>[3x]MRRFGSKFASGLASRCALACPLASAATAPAGASTTSSTSSAQKSFFKTTEMIGYVHSIDGTIATLIPAPGNPGVAYNTIIQIQVSPTTFAAGLVFNLEKDGRIGIILMDNITEVQSGQKVMATGQLLHIPVGAGVLGKVVNPLGHEVPVGLVTRSRRLLDSTLGKVDTGAPNIVSRSPVNYNLLTGFKAVDTMIPIGRGQRELIVGDRQTGKTSIAVSTIINQVRINQQILSKNAVISIYVSIGQRCSNVARIHRLLQSYGALRYTTVMAATAAEPAGLQYLAPYAGVTMGEYFMNRGRHCLCVYDDLSKQAVAYRQISLLLRRPPGREAYPGDVFYLHSRLLERAAMLSPGKGGGSVTALPIVETLSNDVTAYIVTNVISITDGQIYLDTKLFTGGQRPAVNIGLSVSRVGSSAQNAAMKGVAGKLKGILAEYRKLAADSVGGQQVQTIPMIRGARFVALFNQKQPSYFMNAIVSLYACLNGYLDDVKVQYVKFYEYLLVHRDLGIMYGTAKNKFFYMYVQELNYLIRFFTLNSPILHGELEEMLKQHTHLFLQHYQSKMNAIKSEKDVKALKNLLYSCKRAV;>[3x]MLTRFRSAVLRGAVSITGARAASTAPVADHKGRVGHVSQVIGAVVDVHFADGVPPVLTALDVVDKLGRDEPLTLEIVQHLDAHTGRCIAMQTTDLLKLKAKVVSTGGNISVPVGRETLGRIFNVLGDAIDQRGPVGEKLRMPIHAVAPKLADQAAEDAVLTTGIKVIDLILPYCKGGKIGLFGGAGVGKTVIIMELINNVAKGHGGFSVFAGVGERTREGTDLYLEMMQSKVIDLKGESKCVLVYGQMNEPPGARARVAQSALTMAEYFRDVEGQDVLLFIDNIFRFTQANSEVSALLGRIPAAVGYQPTLAEDLGQLQERITSTTKGSITSVQAVYVPADDITDPAPATTFSHLDATTVLDRAVAESGIYPAVNPLECASRIMDPDVISVDHYNVAQDVVQMLTKYRELQDIIAVLGIDELSEEDKLIVDRARKLVKFLSQPFQVAEVFTGMTGHYVQLDDTIDSFSGLLMGTYDQVPEMAFYMVGGINSVLEKAKKMAEEAAELEKMRRARVAQASS;> MSGKLRLYKEKLEGYNRFYSIVKTIKMVTLAKYRAAQGRIRTRDFSLRYTELAFSKPQASRDAVVAAKNALVYIPITTNRGSCGALNSNIVRCIDSVVSSKMVLMPVGKRGIDSFSKLYPDEFRYGIINDMKESMHFGYATFVIENAYEVSKDADRYQVIFNRFVSAGVQRNAVYNIPSYEKWKEDLADAASSDNQKNRYLFANALQNEEEQLIRDFFDFHAALAVLNAVGENELSEQAARLVAVEGQLTNISSLQQRTSSLYNKTRQFGITAALIEILSAMSSLEGNAMKGVRRNKFWEGAVTK;> MFRTFGRRLVSCTLPLLQSAPHDLPEGFEFMEHKVVNKDIHAPHENLETLRLTLTRQDEFLLREEPVKCVTVTGTNGEYGIYPGHAYKIVQLNPSPLTVEYTDGTTKKYFVSGGFAHINNEGSCDVNTVECTLLDDLDLAIAEKELAAQQAALGSAKDDKAKSVVEIRISVIEAVIAALKHH;> MIRRSCALLSSSWRDHGISYLKYLNVCTETLHSTVKESRRAKYERWSKPCYTAQRPDGAGGQETIDKVPIHTKDY;>[3x]MMRRVYSPVFCSVAAARFAATSAAKKYDLFGYEVDTNTAPWIEKIKKCKYYDEAGEVLVNMNVSNCPPDIATYNATLQCIYQSPSKQSTPVDNESKFCAMMDLLEEMQHRNRLKPNEESWTWVMKECVKSGQFRLGYCIQQVMETECKGCPADLVKANEANAQKAKTEGKEHPGHLSQQAGLFDVKVE;>MSAKAAPKTLHQVRNVAYFFAAWLGVQKGYIEKSANDRLWVEHQRKVRQQNVERQQALDSIKLMQQGVRATTPGQLEGVPAELQQLAEAFTK[2x];>[2x]MSSTKCAVACKIMTPLCNAASKVQARSAKKLAALTDAGIQKTISEHNANGTDAAVSSTKRYLAEQRQLFHYRVVRFFDECHYIISGEYFAQYTKVNLIWDLRFLTKLVVLFLIGTVLGRQSIFPPIDPDSPLVEALVTKVNPNY;> MFRRLSSSARAVVAARFYTPPEGLKKLYASDFENSKYPLNIVPSDSVLFAKFLYKAAEEKGNFDNILSDFQKIAAAASKLPIFWERTAVVEKIPEFKQLSEPTFFTLVWMQNNGMLELIQEVAEVYETFVNAKQKKAVAKIFVAPGGEKNVEEARRVAEELHKGLKELADYTLVLKTVVDRTIVKGFAVELAGQYVNKAEGQQKQAGRADEVDYTNLPAPKPQKTVWDDNIETEVLRKYLDGLSQYDMEEAKYGV;>MMRRLALQSSIRRATPFATPLVASTKALNPMCSAITIREASTVAISVQGLHYVGTGLAAIALAGVGLGIGTIFGNLLVACARQPNLTKMLFNYAILGFALTEAIGLFALMLAFLMLFS[10x];> MFLFFFCDLFWLRLLLCMYYCVWSRLCFIVYFNCLMLIFDFLLFCLFDLYLFVGLCLFLLLWFMLFNLYSLILYYCITYLNLYLLFCIVFLLYIAFLFLFCFLCDFFLFNNLLVGDSFMDVFFIRFLLCFLECFSLLCRCLSTFLRLFCNLLSSHFLLLMFFDFFYFIFVFFFYGVFCYWFILFIFVFCFCLLFYVFLYLLDLFAAILQLFIFCNMILQLIMDFLLFLLFV;> MLRRLGANVSNMARPMNKYAVTVSPRRHLEPMSTWYLASWAMVWYYAFFFWMPMVWTDIMVPSFVYNKLPVIHFLQEKRAEQKLRRVLDETYTEWTEELDQAHVTDAITRSLNI;> MRRVSSPNITIQSVRWISGVSPLLYFPPTTTSTTNREDQINKNTNIAIQMIKRYKGEVPPHYTRKSSATIEQVEKEIDALLGGAEKLRKTSTDDQPMDKLTLMERCLRHALWSYHKEEGRYDFDQIGRWVVYTPEDEVKLAQLKREVEAKEKLAALRKRREEEGLPGGPVPRINWPQEYSSFIDREPVVAKRIRYDTLASTTLERDEKQIESTLQQYRRASQDKRLDDLVDLLERFKPVLAREAIMQRLTIKHLEGQLGVWRYMDWCPEVRDRAELEVDITGWQWWSPLEERRLLPVRLRSVNEVREIMSKTQAKKSAEAAERNPIVTQTSTGDNARDRLLKEVLALQARINQRDEVEPSQTEQKKKAHH;> MQGSWSVLKKNCSNFFPGLLAFAQQTQEAYGIWLRIYNRQQKYGPTDFVEQSETFSPDYHKRFHSQDKNMWVDKELCTEVSQKEVARLMTYKLDMWRMAHCAGALLATGGYAIPFGLFWLANDTWVPSSFNLTGEELRAWREAQDLYRYRSAPSYLTDTKWHFDFHAYPWNETQERAWDDLFEKNDVRRDPKVVRPAAEMYDGFIKFELIRRKSLRHLCRSMNIPTFPMLARLCNGTRVRDYWNLAWCEDYMVITQRLHESMTDEELYDYAWRRYLAPYDKNLNREQLMERVEDYFEFLGPDFVAHGKAPNLVILTNYVLGYYNDPAYLEGDISELDKNDYDHLASWGKDAFLRRLEFENGPLRDQVEAHTQRLLAERAAIAKGDNAAAVEGRHTA;> MVLFSTYRSSRLVSKEFLHGPVMRFRALGEYYFQRAWNGTLNWALPGEYRLYAVMIPFIYFYHRWHNDHTLDRDHVEKAMIMRWGGTLEDVRKLSAKDQLRVRCFTDIEKLYSAYGPKDTYLQPPGDTLPGKDFYRKAGGAQAHH;> MSKQLTFISAGATAAVLQSASAIVSKVAGGRVQTKTAKEAGRHAVVVGPETPIGVHTAVTEVPKSAQDPLFSGVSTVVVRAVLPRAAPDSVQLRDALDVYASAGIDTKEEVRSATEAFKKSAEVAVGKAKAKGVKRIVLVVKQASKHNCINELFKKISTETIESAGLTTEVVGTAAVANQLIVNPESLGVVLLNDVAATEQIELAFAGVVGGVSRVYHTVEGGKISAGHSFKSVALAVAQELRELGLSSEADKVEAAASKNPRAVVSAL;> MRRTFISFSAASAAAAAPVTSTKMQTLHKLLTGEVSFKNKAPVKDCNIVHQFGENWATELSAYAKTLPAEQQKIIVRQIARVKLTRYTVAELAAYCGDGPALLDETARAANIEQGVAFVKAKGVEAFEKYVAEESTNANWKPEEAKKFIEDVKAKAK;> MVYTRWKCDRLPVFQLKLFTQEYPMHAAVGIFTIIFLWKHMSHCSEETERKYGWWAGYPYWRDPIARRNETKYKQMIINNDVDITHPKWTGCSVEQLEELSRVV;> MTKYELKMQYFDEWMIRWRKFQTESDWEIEKGRQWWRRFNMAVSGALFCGLVLYTSGTATLKRQYGLPHFFDIGVDGQAKETMLKTLTSRWRYTPQGYGRVLITGVPTYILFVTLEHYRERRRMQQYLQQNTVFGEQMRRLLSTGKIEEYLPVNIKATLPASQQAIYNY;> MLRRSSAALIRRTPVRHSGGELFVRPKLEEIPPADQCRGFFGPLNDSLKFLRLLDIKWMMNRAVAMRREYLIATPTLFTFIWMFTWKGAVIYFWGDRAPPRRMDWNTEETGRLPLGFKPTPAPL;> MLRKTPLFAMATTRKALVGNGPTFSTGGECMNTCDIQNAFPMNDRGVRSSSPFQEPNTAIYDSYLAWTYFQPMDVHIEKLPAPEAKYYQRHTKKPWDVSSTELTEIQSRKKYFQTLGYLVAFIYLYFLMPKEKSFSGLSGPDGHWIMLPKGRPELF;> MSSGFHFHDVSNDAIKGMPPSEALHKHLENAQLAHRICLAKALKAGEPPVEKCALTWGEVLIRYQAWSEYRPPFQDSVAQAKYKKYWSKKRQEEDDKNPFK;> MLRRLVPRVMMAPMGGATALCTSRGYNMLVFRDPKRRPQLSEEERAKVVVNQAEWPEEFKDFDPDDPYKNSPEIIKGMSSWNLFLWGVECAFIYQFYELVFPKSI;> MTENIEAVMSDFWSNPADHFRPNLKALTLYAERQHYVDRWLHVKERWLAPWYLPWWSPLFQLGTWYSQRSRNLFLVENHLSYRPYKFRRNDEDRNNPY;> MLLGGFVPRRFSQFNRDPCWMFFIFSVGFWLGEYPAMMIKYNARDLVYDPHRYVWSHHDDHH

Mitochondrial ATP synthase consists of the soluble F1 and membrane-bound Fo subcomplexes and occurs in dimers that assemble into oligomers to induce the formation of inner-membrane folds, called cristae. Dissociation of ATP synthase dimers into monomers results in the loss of native cristae architecture and impairs mitochondrial function. Here, we report cryo-EM structures of the intact ATP synthase dimer from Trypanosoma brucei in ten different rotational states. Although overall dimer architecture varies among eukaryotes, we find that subunit-g together with subunit-e form an ancestral oligomerization motif, which is shared between the trypanosomal and mammalian lineages.

To describe the conformational space of the T. brucei ATP synthase, we resolved ten distinct rotary substates, which were refined to 3.5–4.3 Å resolution. The three main states (1–3) result from three ~120° rotation steps of the rotor relatively to the static Fo. We identified five (1a–1e), four (2a–2d), and one classes of the respective main states. Throughout all the identified substeps of the rotational state 1 (classes 1a to 1e) the rotor turns by ~33°, which corresponds approximately to the advancement by one subunit-c of the c10-ring. While rotating along with the rotor, the F1 headpiece lags behind, advancing by only ~13°. However, due to its large, rigid peripheral stalk, the Polytomella ATP synthase mainly displays rotational substeps, whereas the Trypanosoma F1 also displays a tilting motion of ~8° revealed by rotary states 1a and 1b. In all classes F1 is in a similar conformation, corresponding to the catalytic dwell, observed previously also in the crystal structure of T. brucei F1-ATPase13.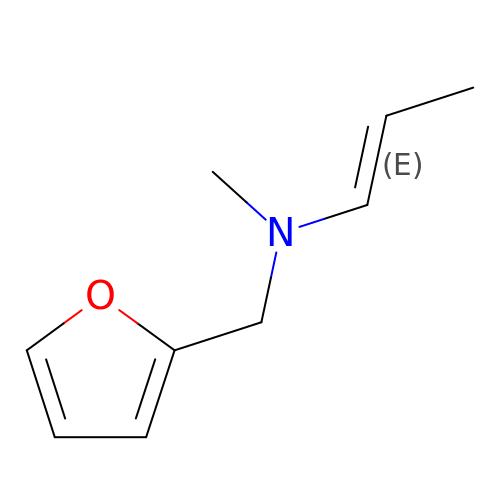(~{E})-~{N}-(furan-2-ylmethyl)-~{N}-methyl-prop-1-en-1-amine | C9 H13 N O | DBDADMSUVDNQKI-ZZXKWVIFSA-N> GPEKDPIEDINSPEHIQRRLSLQLPILHHAYLPSIGG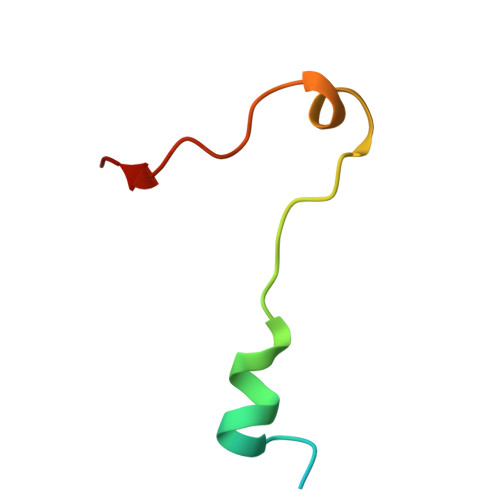VDAS> MLKRFPTPILKVYWPFFVAGAAVYYGMSKAADLSSNTKEFINDPRNPRFAKGGK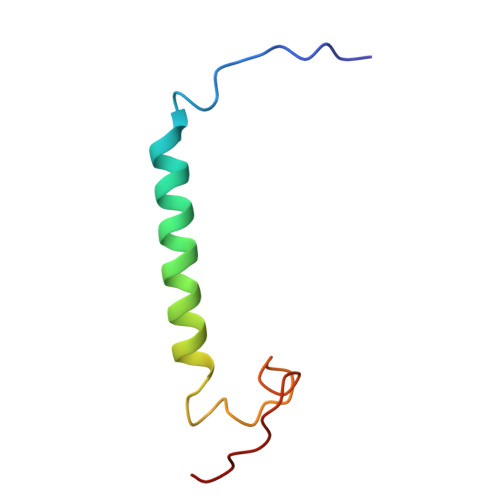FVEVD> GVTFDDGAYTGIREINFEYNSETAIGGLRVTYDLNGMPFVAEDHKSFITGFKPVKISLEFPSEYIVEVSGYVGKVEGYTVIRSLTFKTNKQTYGPYGVTNGTPFSLP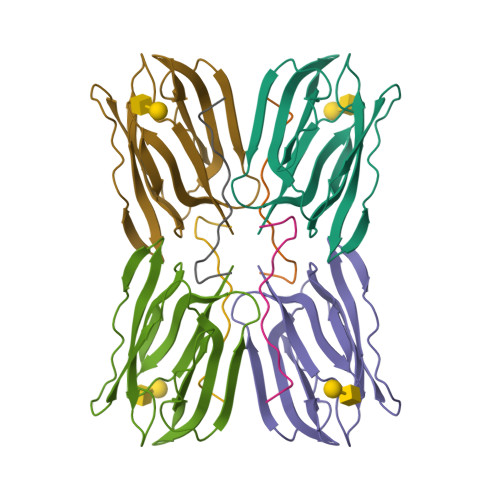IENGLIVGFKGSIGYWLDYFSIYLSL;> GRNGKSQSIIVGPWGDRVTN>[3x]SLRSDLINALYDENQKYDVCGIISAEGKIYPLGSDTKVLSTIFELFSRPIINKIAEKHGYIVEEPKQQNHYPDFTLYKPSEPNKK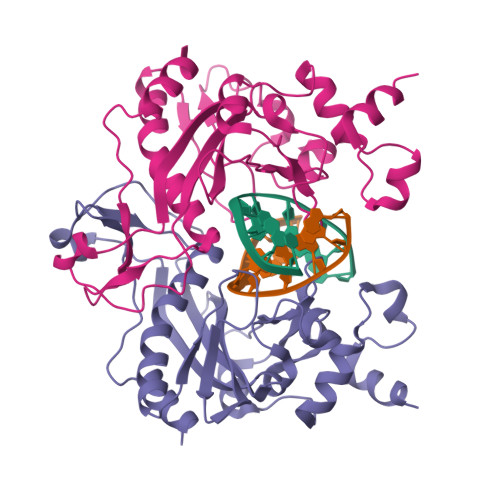IAIDIKTTYTNKENEKIKFTLGGYTSFIRNNTKNIVYPFDQYIAHWIIGYVYTRVATRKSSLKTYNINELNEIPKPYKGVKVFLQDKWVIAGDLAGSGNTTNIGSIHAHYKDFVEGKGIFDSEDEFLDYWRNYERTSQLRNDKYNNISEYRNWIYRGRK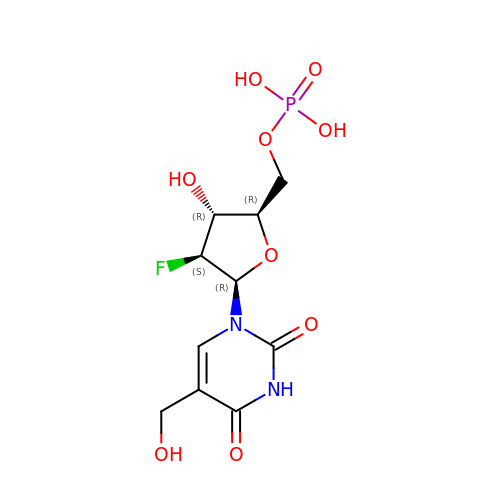1-(2-deoxy-2-fluoro-5-O-phosphono-beta-D-arabinofuranosyl)-5-(hydroxymethyl)pyrimidine-2,4(1H,3H)-dione | C10 H14 F N2 O9 P | MCTFWHKMGAFQIE-JVZYCSMKSA-N Here, we have studied a potential GH8 xylanase from the shipworm symbiont T. turnerae, the genome sequence of which unveiled a treasure chest of carbohydrate-active enzymes. We have shown that TtGH8 is a single-domain endo-xylanase with six catalytically relevant subsites that hydrolyses X6 to yield predominantly xylotriose. CAZY GH8 enzymes act with inversion of anomeric configuration and thus feature two essential catalytic residues: a base to activate the water for nucleophilic attack and an acid to protonate the leaving group for departure. Intriguingly, TtGH8 shows the highest activity on mixed-linkage β-1,3,β-1,4 xylans, which may reflect a genuine biological adaption to, or at least an accommodation of, these marine substrates.

Given its possible relevance to xylan degradation and perhaps even marine colonization of wood, DNA encoding the predicted catalytic domain (residues 41–436) of the GH8 enzyme of the bacterium (TtGH8; locus tag TERTU_4506) was cloned into an E. coli expression vector. E. coli containing the recombinant plasmid produced high levels of soluble TtGH8, which was purified using nickel-affinity chromatography and gel-filtration chromatography. In order to provide molecular insight into its catalytic properties the three-dimensional structure of TtGH8 was determined. The three-dimensional structure of TtGH8, determined to 1.5 Å resolution, reveals intimate details of the substrate-binding sites and the distortions of xylose within the catalytic centre. PDBeFold analysis reveals that TtGH8 shares close structural similarity to the reducing-end xylose-releasing exo-oligoxylanase from B. halodurans C-125. TtGH8 shares 43% sequence identity, overlaying 344 Cα atoms with an r.m.s.d. of 1.1 Å, a Q score of 0.7 and a Z score of 15.9. The next closest match is the cold-adapted GH8 xylanase from Pseudoalteromonas haloplanktis with 35% sequence identity, an r.m.s.d. of 1.4 Å over 341 Cα atoms, a Q score of 0.6 and a Z score of 14.7.

> GPAAGAVATGEYRNLFAEIGKSEIDIQRKIDEAFQHLFYGDAKDAAVYYQAGGNENGPLAYVYDVNSNDVRSEGMSYGMMITVQMDKKAEFDAIWNWAKTYMYQDSPTHPAFGYFAWSMRRDGVANDDMPAPDGEEYFVTALYFAAARWGNGEGIFNYQQEADTILSRMRHRQVITGPTNRGVMTATNLFHPEEAQVRFTPDINNADHTDASYHLPSFYEIWARVAPQEDRAFWAKAADVSRDYFAKAAHPVTALTPDYGNFDGTPWAASWRPESVDFRYDAWRSVMNWSMDYAWWGKDSGAPARSDKLLAFFETQEGKMNHLYSLDGKPLGGGPTLGLISMNATAAMAATDPRWHNFVEKLWQQQPPTGQYRYYDGVLYLMALLHCAGEYKAWIPDGE>MKKWANLDSGESEDPPHEDSCPDPPDGDPNSKQSPAKPHIFSTTKSRTRLFGKGDSEEASPMDCSYEEGELASCPTITVSSVVIIQRPGDALTCARQLSQDSVSAGAEKPLKLYDRRSIFDAVAQNNCQELESLLPFLQKSRKRLTDSEFKDPETGKTCLLKAMLNLHNGQNDTISLLLDIARQTDSLKEFVNASYTDSYYKGQTALHIAIERRNMALVTLLVENGADVQAAANGDFFKKTKGRPGFYFGELPLSLAACTNQLAIVKFLLQNSWQPADISARDSVGNTVLHALVEVADNTADNTKFVTSMYNEILILGAKLHPTLKLEELINKKGLTPLALAASSGKIGVLAYILQREIQEPECRHLSRKFTEWAYGPVHSSLYDLSCIDTCEKNSVLEVIAYSSSETPNRHDMLLVEPLNRLLQDKWDRFVKRIFYFNFFVYCLYMIVFTTAAYYRPVDGLPPYKLKNTVGDYFRVTGEILSVSGGVYFFLRGIQYFLQRRPSMKTLFVDSYSEMLFFVQSLFMLGSVVLYFSHRKEYVASMVFSLAMGWTNMLYYTRGFQQMGIYAVMIEKMILRDLCRFMFVYLVFLFGFSTAVVTLIEDGKNYSEPAEYTSHRWRAPGCRPPDSYNSLYSTCLELFKFTIGMGDLEFTENYDFKAVFIILLLAYVILTYILLLNMLIALMGETVNKIAQESKNIWKLQRAITILDTEKSFLKCMRKAFRSGKLLQVGYTPDGKDDYRWCFRVDEVNWTTWNTNVGIINEDPGNCE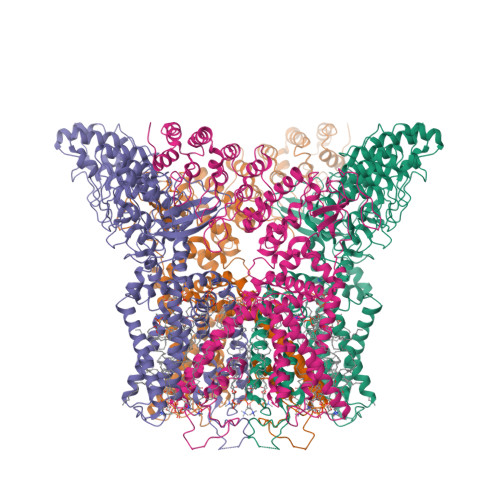GVKRTLSFSLRSGRVSGRNWRNFALVPLLRDASTRDRHHAQPEEVHLKHFAGSLKPEDAEVFKDSMAPGEKLPVR[4x]>GCAGACUUAAGUCUG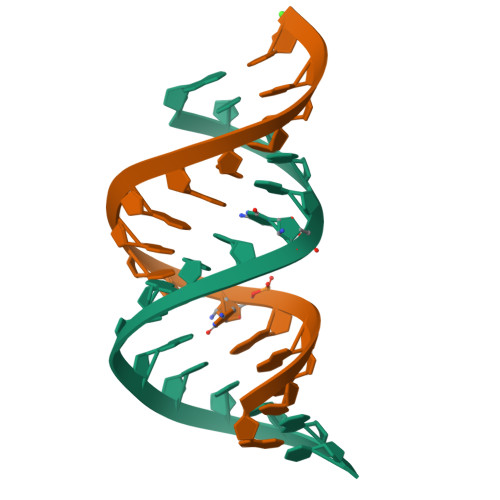C[3x]> AIGEFMVSLPRMVYPQPKVLTPCRKDVLVVTPWLAPIVWEGTFNIDILNEQFRLQNTTIGLTVFAIKKYVAFLKLFLETAEKHFMVGHRVHYYVFTDQPAAVPRVTLGTGRQLSVLEVRAYKRWQDVSMRRMEMISDFCERRFLSEVDYLVCVDVDMEFRDHVGVEILTPLFGTLHPGFYGSSREAFTYERRPQSQAYIPKDEGDFYYMGAFFGGSVQEVQRLTRACHQAMMVDQANGIEAVWHDESHLNKYLLRHKPTKVLSPEYLWDQQLLGWPAVLRKLRF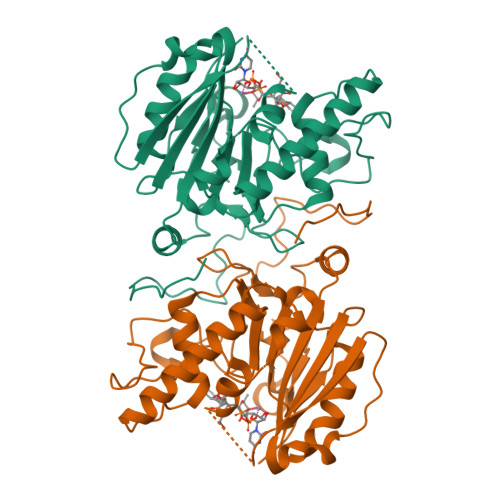TAVPKNHQAVRNPE> DVSTSYLRHNEINEYLQTLSQKYPSLVSVEEAGTSYEGRSIKTITINKKPGNAVVFLDAGIHAREWIAPATALYAIEQLVEHSSENQEVLSNLTWVIMPVVNPDGYEFSHETDRFWRKTRKPTGKSCKGTDGNRNFDYHWGEVGASTQACADTFRGETAFSEPETRAVRDAVMKLKGSCKFYLSLHSYGNYILYPWGWTSKLPETWEAIDEVAQAGAEAIKQSTGSRYTVGSSTNVLYAAAGGSDDWAFAVAEVPISITMELPGGGNGGFNPPPSSIEKIVNESWVGI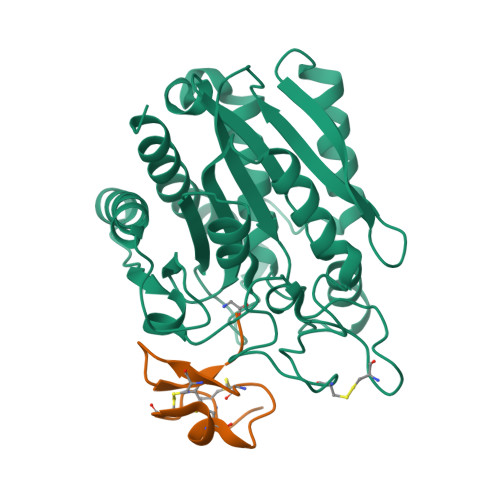KAMALKVAQMF;> HADPICNKPCKTHDDCSGAWFCQACWNSARTCGPYV Previous studies showed that proper introduction of disulfide bonds could stabilize the flexible region of target proteins and reduce the conformational entropy by locking the protein into single desired conformation. Here we developed a comprehensive disulfide bond prediction algorithm that not just increased the success rate of predictions but also improved the quality of crystallized target proteins. We applied our method on two proteins which were previously determined to high resolution and frequently used as fusion partners for GPCR crystallization, cytochrome b562 (BRIL) and Flavodoxin, and verified our prediction by solving the crystal structures of the wild type (WT) proteins and mutants. The theoretical and experimental results both indicated that with relatively lower values of conformational entropy, proteins would be more stable and readily crystallized to higher diffraction resolution.

The continued disulfide omitted electron densities of the side chains suggested that the disulfide bonds are successfully formed in all crystallized mutants, which are T9C-A36C, A20C-Q25C, V16C-A29C, and K27C-A79C in BRIL and N14C-C93, A43C-L74C, and C102-R125C in Flavodoxin, respectively. The WT and disulfide engineered Flavodoxin structures were determined to high-resolution of 1.20–1.55 Å with B-factors in the range of 16.15–19.24 Å2. For Flavodoxin, the reduced B-factors for R125C mutant indicated that the disulfide bond further stabilizes the structure.

> SAKALIVYGSTTGNTEYTAETIARELADAGYEVDSRDAASVEAGGLFEGFDLVLLGCSTWGDDSIELQDDFIPLFDSLEETGAQGRKVACFGCGDSSWEYFCGAVDAIEEKLKNLGAEIVQDGLCIDGDPRAARDDIVGWAHDVRGAI> MLPKFDPTNQKACLSLLEDLTTNVKQIQDSVLEAILSRNAQTEYLRGFLNGQVDKQNFKKNVPVVTYEDIRSYIDRIANGEPSDLICDRPISVLLTSSGTSGGVPKLIPLTTEDLEQRISFSSLYAPLLYKHIDGLSEGKSLIFYFVTRESKTANGLMVRTMVTSFLKSIKQTNSFLWDSLQVSPHAITTCADTTQSMYCQLLCGLLERDNVARLGAPFASSFLKVIKFLEDHWPELCSNIRTGRLSDWITDATCTSGIGKFLTAPNPELASLIEQECSKTSWEAILKRLWPKAKCIESIITGTMAQYIPLLEFYSGGLPLTSSFYGSSECFMGVNFNPLCKPSDVSYTIIPCMGYFEFLEVEKDHQEAGHDPTEKPVVVDLVDVKIGHDYEPVVTTFSGLYRYRVGDVLRATGFYNNAPHFCFVGRQKVVLSIDMDKTYEDDLLKAVTNAKLLLEPHDLMLMDFTSRVDSSSFPGHYVIYWELGSKVKDAKFEPNRDVMEECCFTVEESLDAVYRKGRKNDKNIGPLE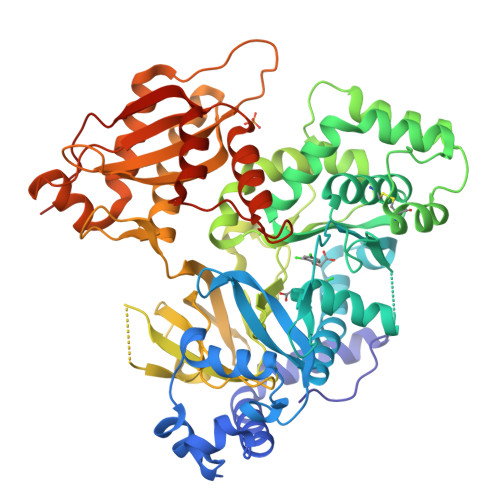IKVVKPGAFDELMNFFLSRGSSVSQYKTPRSVTNEEALKILEANVISEFLSRKIPSWELHELHSGR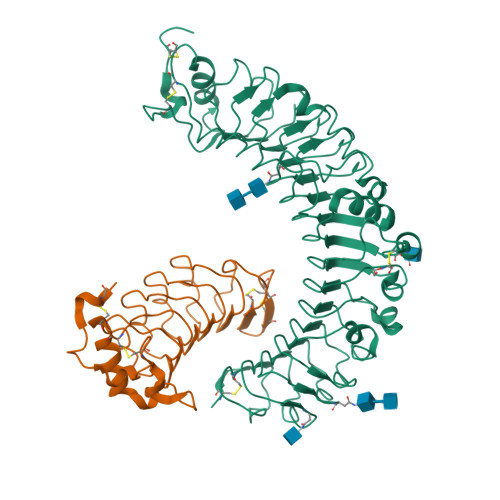>ADPGTSECSVIGYNAICINRGLHQVPELPAHVNYVDLSLNSIAELNETSFSRLQDLQFLKVEQQTPGLVIRNNTFRGLSSLIILKLDYNQFLQLETGAFNGLANLEVLTLTQCNLDGAVLSGNFFKPLTSLEMLVLRDNNIKKIQPASFFLNMRRFHVLDLTFNKVKSICEEDLLNFQGKHFTLLRLSSITLQDMNEYWLGWEKCGNPFKNTSITTLDLSGNGFKESMAKRFFDAIAGTKIQSLILSNSYNMGSSFGHTNFKDPDNFTFKGLEASGVKTCDLSKSKIFALLKSVFSHFTDLEQLTLAQNEINKIDDNAFWGLTHLLKLNLSQNFLGSIDSRMFENLDKLEVLDLSYNHIRALGDQSFLGLPNLKELALDTNQLKSVPDGIFDRLTSLQKIWLHTNPWDCSCPRIDYLSRWLNKNSQKEQGSAKCSGSGKPVRSIICPTSASLVPR[2x];>GGHHHHHHGSENLYFQGACPSQCSCSGTTVDCSGKSLASVPTGIPTTTQVLGLSSNQITKLEPGVFDSLVNLQILVLYQNQLTTLPAGVFDRLINLKELYFSNNQLTSLPAGVFDKLTQLTRLELQTNQLKSIPRGAFDNLKSLTNIYLFNNPWDCECSDILYLKNWIVQHASIVNPDGHGGVDNVKCSGTNTPVRAVTEASTSPSKCP[2x]>MGSSHHHHHHSSGLVPRGSGGYEIPARLRTLHNLVIQYASQGRYEVAVPLCKQALEDLEKTSGHDHPDVATMLNILALVYRDQNKYKDAAHLLNDALAIREKTLGKDHPAVAATLNNLAVLYGKRGKYKEAEPLCKRALEIREKVLGKFHPDVAKQLSNLALLCQNQGKAEEVEYYYRRALEIYATRLGPDDPNVAKTKNNLASCYLKQGKYQDAETLYKEILTRAHEKEFGSVNGENKPIWMHAEEREESKDKRRDSAPYGEYGSWYKACKVDSPTVNTTLRSLGALYRRQGKLEAAHTLEDCASR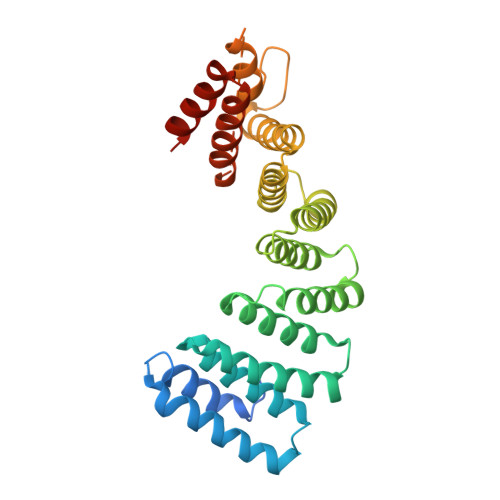SRKQGLD[3x]> SDEADEAYSVTEQLTMTGINRIRQKINAHGIPVYLCEACGNPIPE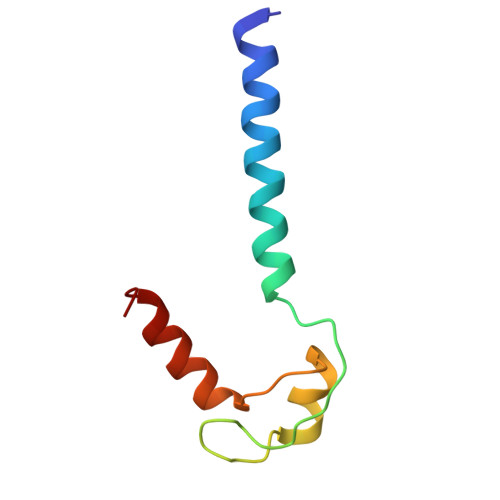ARRKIFPGVTLCVECQAYQERQRKHYA(1E,10S)-1-(3,5-dihydroxyphenyl)-10-hydroxyundec-1-en-6-one 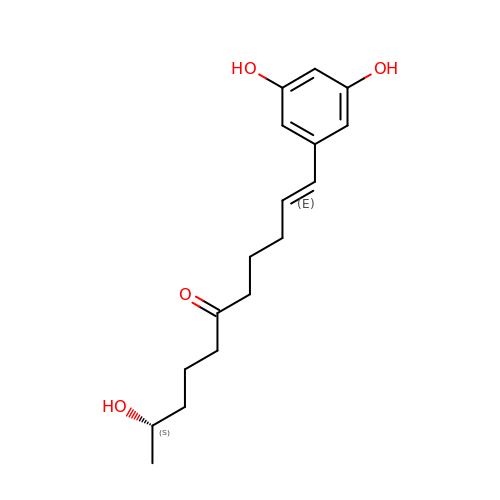| C17 H24 O4 | TVXRLKRGDWQGQV-MXPWBENCSA-N> XSI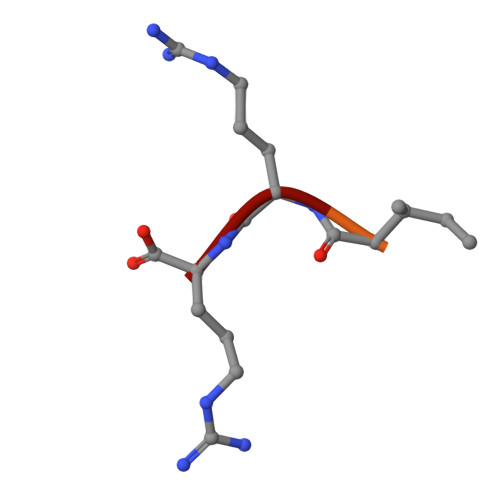IRR9-AMINO-(N-(2-DIMETHYLAMINO)BUTYL)ACRIDINE-4-CARBOXAMIDE 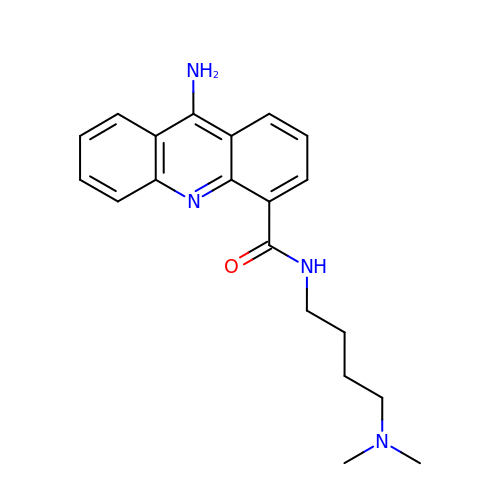| C20 H24 N4 O | AMFZHKPIXJORQY-UHFFFAOYSA-N>AMYSTNAYAELAGPPKIFCKSVSKDPDFRLKQIDYVIPVQQDRSICMNNPLLDISDGFFTYIHYEGINSCKKSDSFKVLLSHGEIVDRGDYRPSLYLLSSHYHPYSMQVINCVPVTCNQSSFVFCHISNNTKTLDNSDYSSDEYYITYFNGIDRPKTKKIPINNMTADNRYIHFTFSGGGGVCLGEEFIIPVTTVINTDVFTHDYCESFNCSVQTGKSLKEICSESLRSPTNSSRYNLNGIMIISQNNMTDFKIQLNGITYNKLSFGSPGRLSKTLGQVLYYQSSMSWDTYLKAGFVEKWKPFTPNWMNNTVISRPNQGNCPRYHKCPEICYGGTYNDIAPLDLGKDMYVSVILDSDQLAENPEITVFNSTTILY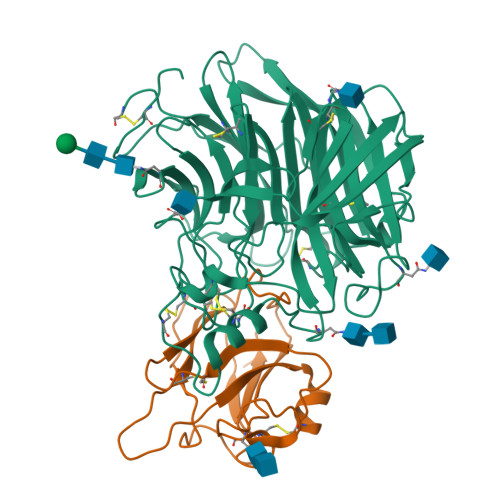KERVSKDELNTRSTTTSCFLFLDEPWCISVLETNRFNGKSIRPEIYSYKIPKYC[2x];>AKNLEPVSWSSLNPKFLSGKGLVIYPKIGDKLDIICPRAEAGRPYEYYKLYLVRPEQAAACSTVLDPNVLVTCNKPHQEIRFTIKFQEFSPNYMGLEFKKYHDYYITSTSNGSLEGLENREGGVCRTRTMKIVMKVGQDPNA[2x]> MRVEALGKVAPLPQAQTPVSLNEASLEELMALPGIGPVLARRIVEGRPYARVEDLLKVKGIGPATLERLRPY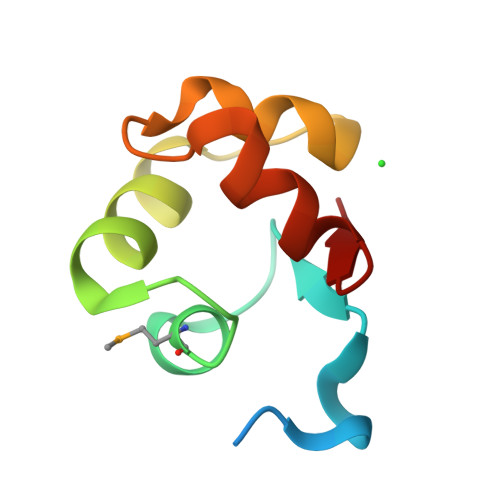LRP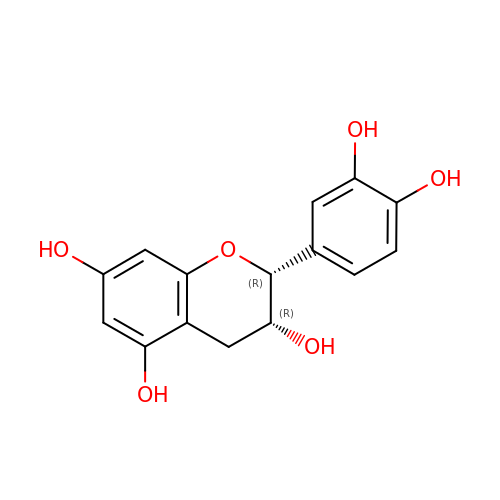(2R,3R)-2-(3,4-dihydroxyphenyl)-3,4-dihydro-2H-chromene-3,5,7-triol | C15 H14 O6 | PFTAWBLQPZVEMU-UKRRQHHQSA-N>[2x]SYHLDTTAPPPTNLSTLPNNTLFHLWRPRAHILPAEGQIGDPCAHYTDPSTGLFHVGFLHDGDGIAGATTANLATYTDTSDNGSFLIQPGGKNDPVAVFDGAVIPVGVNNTPTLLYTSVSFLPIHWSIPYTRGSETQSLAVARDGGRRFDKLDQGPVIADHPFAVDVTAFRDPFVFRSARLDVLLSLDEEVARNETAVQQAVDGWTEKNAPWYVAVSGGVHGVGPAQFLYRQNGGNASEFQYWEYLGEWWQEATNSSWGDEGTWAGRWGFNFETGNVLFLTEEGHDPQTGEVFVTLGTEGSGLPIVPQVSSIHDMLWAAGEVGVGSEQEGAKVEFSPSMAGFLDWGFSAYAAAGKVLPASSAVSKTSGVEVDRYVSFVWLTGDQYEQADGFPTAQQGWTGSLLLPRELKVQTVENVVDNELVREEGVSWVVGESDNQTATLRTLGITIARETKAALLA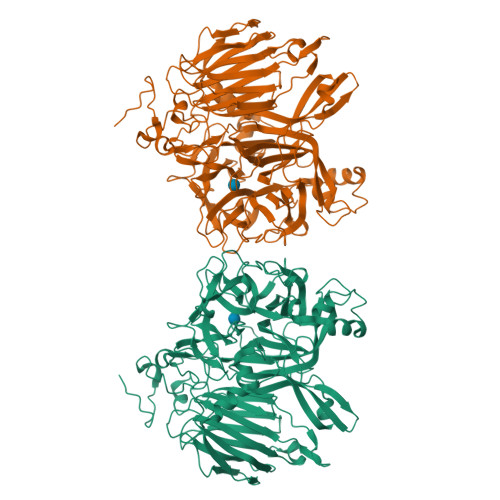NGSVTAEEDRTLQTAAVVPFAQSPSSKFFVLTAQLEFPASARSSPLQSGFEILASELERTAIYYQFSNESLVVDRSQTSAAAPTNPGLDSFTESGKLRLFDVIENGQEQVETLDLTVVVDNAVVEVYANGRFALSTWARSWYDNSTQIRFFHNGEGEVQFRNVSVSEGLYNAWPER> SLNAKKIRLENYAMKMRLYPSPTQAEQMDKMFLALRLAYNMTFHEVFQQNPAVCGDPDEDGNVWPSYKKMANKTWRKALIDQNPAIAEAPAAAITTNNGLFLSNGQKAWKTGMHNLPANKA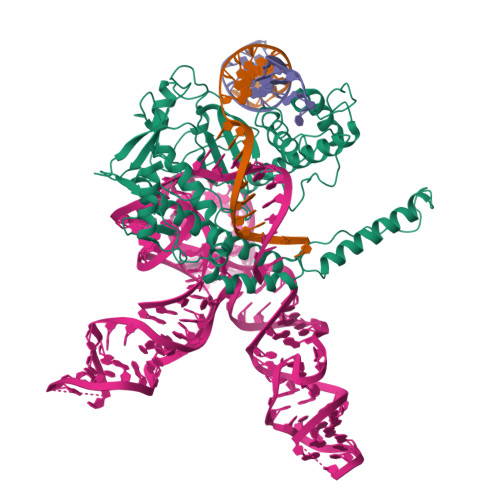DRKDFRFYSLSKPRRSFAVQIPPDCIIPSDTNQKVARIKLPKIDGAIKARGFNRKIWFGPDGKHTYEEALAAHELSNNLTVRVSKDTCGDYFICITFSQGKVKGDKPTWEFYQEVRVSPIPEPIGLDVGIKDIAILNTGTKYENKQFKRDRAATLKKMSRQLSRRWGPANSAFRDYNKNIRAENRALEKAQQDPGSSGVGPEAPVLKSVAQPSRRYLTIQKNRAKLERKIARRRDTYYHQVTAEVAGKSSLLAVETLRVKNMLQNHRLAFALSDAAMSDFISKLKYKARRIQVPLVAIGTFQPSSQTCSVCGSINPAVKNLSIRVWTCPNCGTRHNRDINAAKNILAIAQNMLEKKV>MKDSEIFTVNGILGESVTFPVNIQEPRQVKIIAWTSKTSVAYVTPGDSETAPVVTVTHRNYYERIHALGPNYNLVISDLRMEDAGDYKA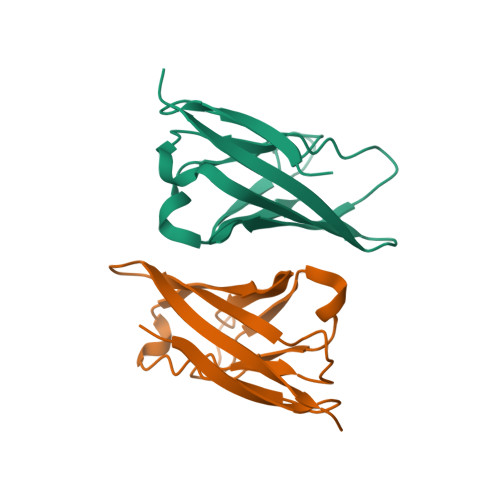DINTQADPYTTTKRYNLQIYRR[6x]> MKRVAQRVKEQMDTNQREYYLREQMKAIQKELGGEDGLSDLEALRKKIEEVGMPEAVKTKALKELDRLERMQQGSPEATVARTYLDWLTEVPWSKA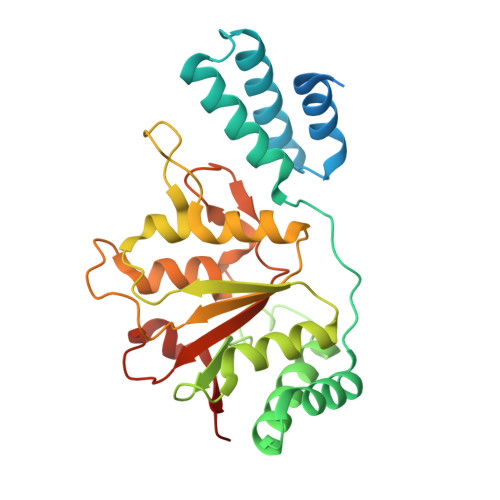DPEVLDINHTRQVLDEDHYGLKDVKERILEYLAVRQLTQGLDVRNKAPILVLVGPPGVGKTSLGRSIARSMNRKFHRISLGGVRDEAEIRGHRRTYIGAMPGKLIHAMKQVGVINPVILLDEIDKMSSDWRGDPASAMLEVLDPEQNNTFTDHYLDVPYDLSKVFFITTANTLQTIPRPLLDRMEVIEIPGHHHHHH>LINLKYSVEEEQRAGTVIANVAKDAREAGFALDPRQASAFRVVSNSAPHLVDINPSSGLLVTKQKIDRDLLCRQSPKCIISLEVMSSSMEICVIKVEIKDLNDNAPSFPAAQIELEISEAASPGTRIPLDSAYDPDSGSFGVQTYELTPNELFGLEIKTRGDGSRFAELVVEKSLDRETQSHYSFRITALDGGDPPRLGTVGLSIKVTDSNDNNPVFSESTYAVSVPENSPPNTPVIRLNASDPDEGTNGQVVYSFYGYVNDRTRELFQIDPHSGLVTVTGALDYEEGHVYELDVQAKDLGPNSIPAHCKVTVSVLDTNDNPPVINLLSVNSELVEVSESAPPGYVIALVRVSDRDSGLN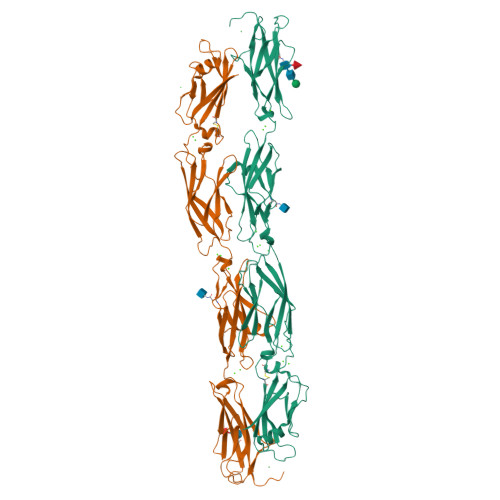GRVQCRLLGNVPFRLQEYESFSTILVDGRLDREQHDQYNLTIQARDGGVPMLQSAKSFTVLITDHHHHHH[3x]>[2x]MNINQEQLLMFQAVMETGSFSAAARKLGKVPSAVSMSIANLEIDLNLTLFERKGREPTPTAEARVLYEKTAQLLIEMNQWKQHAHALSTGLEPNLTIVVVSELLHTNWTDYVCLLESRFPDLQINIVSAPQEDALQMLLDGSAQLALMFEREHLDNREQFVELKREALIPVISKTHPLASQEHVSYEQILGTRQIVVASRDETLKPELLFSKHYWRTDNHHSACLMILRNLGWGVLP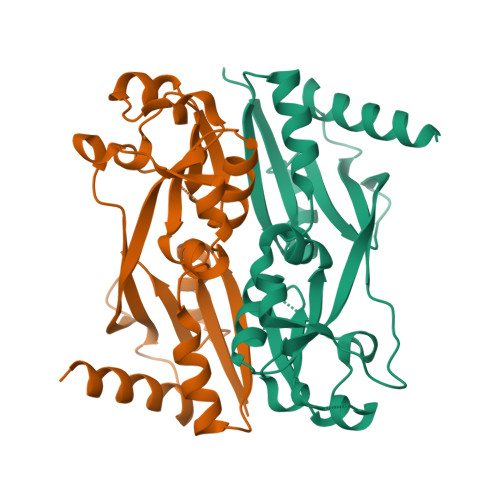QEMFKENPELNNKLKALDVFDFTPRFEYYVDLVWSRESELGAAARFLIDYIRNKRMQPAP>[2x]AAQPARRAVRSSRRHHHHHHGSGLEVLFQGPTPGTKPPECPDFDPPRQENETWWLCDCFMATCKYNNTVEIVKVECEPPPMPTCSNGLQPVRVEDPDGCCWHWECDCYCTGWGDPHYVTFDGLYYSYQGNCTYVLVEEISPSVDNFGVYIDNYHCDPNDKVSCPRTLIVRHETQEVLIKTVHMMPMQVQVQVNRQAVALPYKKYGLEVYQSGINYVVDIPELGVLVSYNGLSFSVRLPYHRFGNNTKGQCGTCTNTTSDDCILPSGEIVSNCEAAADQWLVNDPSKPHCPHSSSTTKRPAVTVPGGGKTTPHKDCTPSPLCQLIKDSLFAQCHALVPPQHYYDACVFDSCFMPGSSLECASLQAYAALCAQQNICLDWRNHTHGACLVECPSHREYQACGPAEEPTCKSSSSQQNNTVLVEGCFCPEGTMNY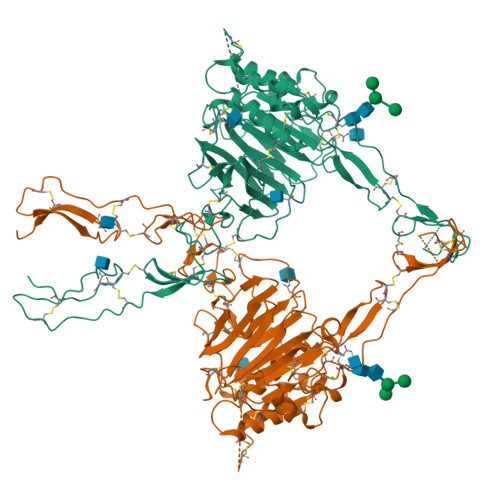APGFDVCVKTCGCVGPDNVPREFGEHFEFDCKNCVCLEGGSGIICQPKRCSQKPVTHCVEDGTYLATEVNPADTCCNITVCKCNTSLCKEKPSVCPLGFEVKSKMVPGRCCPFYWCESKGVCVHGNAEYQPGSPVYSSKCQDCVCTDKVDNNTLLNVIACTHVPCNTSCSPGFELMEAPGECCKKCEQTHCIIKRPDNQHVILKPGDFKSDPKNNCTFFSCVKIHNQLISSVSNITCPNFDASICIPGSITFMPNGCCKTCTPRNETRVPCSTVPVTTEVSYAGCTKTVLMNHCSGSCGTFVMYSAKAQALDHSCSCCKEEKTSQREVVLSCPNGGSLTHTYTHIESCQCQDTVCGLPTGTSRRARRSPRHLGSG> MLSEQQIKEKLDSVPIYLVTNEKGLPLSRPLPNAPNGQKAGGSITGAYMSRQEAQAFINELRNAKNKDP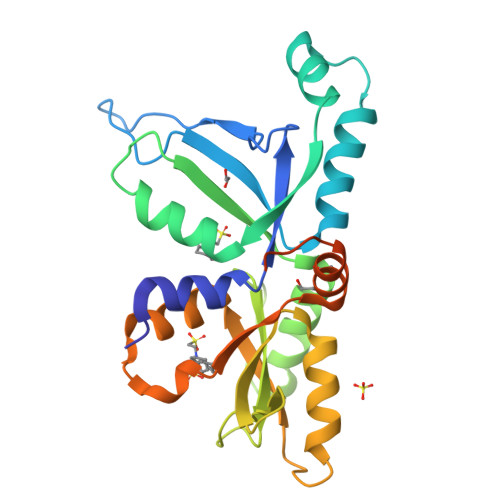KMQEIVKSLQVTAVPLGVIYQQLQQTKKDPNRLLFAFKPVDQEIKGAMDLLRQSGQQVNQFKSVPMFAVRFAPDQGYVPIKVGTGNEQVVPLFLSKQDAQGLLGQVKPKHPKADIQVLDIDGVLQTLQDKNDTWLNQVVLVPSPESREYIRTLPKPPNTPAAPNRNNNNSRPGAKLEHHHHHH> DI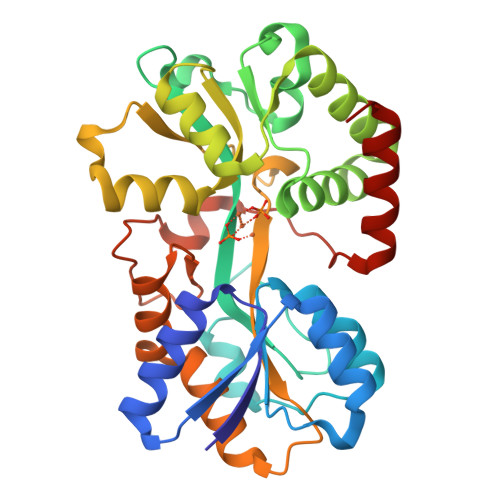TVYNGQAKEAATAVAKAFEQETGIKVTLNSGKSEQLAGQLKEEGDKTPADVFYTEQTATFADLSEAGLLAPISEQTIQQTAQKGVPLAPKKDWIALSGRSRVVVYDHTKLSEKDMEKSVLDYATPKWKGKIGYVSTSGAFLEQVVALSKMKGDKVALNWLKGLKENGKLYAKNSVALQAVENGEVPAALINNYYWYNLAKEKGVENLKSRLYFVRHQDPGALVSYSGAAVLKASKNQAEAQKFVDFLASKKGQEALVAARAEYPLRADVVSPFNLEPYEKLEAPVVSATTAQDKEHAIKLIEEAGLK> MACAAARSPAEQDRFICIYPAYLNNKKTIAEGRRIPISKAVENPTATEIQDVCSAVGLNVFLEKNKMYSREWNRDVQYRGRVRVQLKQEDGSLCLVQFPSRKSVMLYAAEMIPKLKTRTQKTGGGDQSLQQGEGSKKGKGKKKK;> MASADSRRLGDGDGAGGAFQPYLDSLRQELQQRDPTVLSVVVALLAVLLTLVFWKLVRSRRSSQRAVLLLGLCDSGKTLLFVRLLTGHYRDTQTSITDSSATYRVNNNRGNSLTLIDLPGHESLRLQFLERFKTSARAVVFVVDSAAFQREVKDVAEFLYQVLIDSMSLKNTPSFLIACNKQDIAMAKSAKLIQQQLEKELNTLRVTRSAAPSTLDSSSTAPAQLGKKGKEFEFSQLPLKVEFLECSAKGGRGDPGSADIQDLEKWLAKIA;> MVLADLGRKITSALRSLSNATIINEEVLNAMLKEVCTALLEADVNIKLVKQLRENVKSAIDLEEMASGLNKRKMIQHAVFKELVKLVDPGVKAWTPTKGKQNVIMFVGLQGSGKTTTCSKLAYYYQRKGWKTCLICADTFRAGAFDQLKQNATKARIPFYGSYTEMDPVIIASEGVEKFKNENFEIIIVDTSGRHKQEDSLFEEMLQVANAIQPDNIVYVMDASIGQACEAQAKAFKDKVDVASVIVTKLDGHAKGGGALSAVAATKSPIIFIGTGEHIDDFEPFKTQPFISKLLGMGDIEGLIDKVNELKLDDNEALIEKLKHGQFTLRDMYEQFQNIMKMGPFSQILGMIPGFGTDFMSKGNEQESMARLKKLMTIMDSMNDQELDSTDGAKVFSKQPGRIQRVARGSGVSTRDVQELLTQYTKFAQMVKKMGGIKGLFKGGDMSKNVSQSQMAKLNQQMAKMMDPRVLHHMGGMAGLQSMMRQFQQGAAGNMKGMMGFNNM;> MLDFFTIFSKGGLVLWCFQGVSDSCTGPVNALIRSVLLQERGGNNSFTHEALTLKYKLDNQFELVFVVGFQKILTLTYVDKLIDDVHRLFRDKYRTEIQQQSALSLLNGTFDFQNDFLRLLREAEESSKIRAPTTMKKFEDSEKAKKPVRSMIETRGEKPKEKAKNSKKKGAKKEGSDGPLATSKAVPAEKSGLPVGPENGVELSKEELIRRKREEFIQKHGRGLEKSSKSKSEAPKEKGKKAPRVWELGGCANKEVLDYSTPTTNGAPEAALSEDINLIRGTGPGGQLQDLDCSSSDDEGAAQNSTKPSSTKGTLGGMFGMLKGLVGSKSLSREDMESVLDKMRDHLIAKNVAADIAVQLCESVANKLEGKVMGTFSTVTSTVKQALQESLVQILQPQRRVDMLRDIMDAQRRQRPYVVTFCGVNGVGKSTNLAKISFWLLENGFSVLIAACDTFRAGAVEQLRTHTRRLSALHPPEKHGGRTMVQLFEKGYGKDAAGIAMEAIAFARNQGFDVVLVDTAGRMQDNAPLMTALAKLITVNTPDLVLFVGEALVGNEAVDQLVKFNRALADHSMAQTPRLIDGIVLTKFDTIDDKVGAAISMTYITSKPIVFVGTGQTYCDLRSLNAKAVVAALMKA;> MASGGSGGVSVPALWSEVNRYGQNGDFTRALKTVNKILQINKDDVTALHCKVVCLIQNGSFKEALNVINTHTKVLANNSLSFEKAYCEYRLNRIENALKTIESANQQTDKLKELYGQVLYRLERYDECLAVYRDLVRNSQDDYDEERKTNLSAVVAAQSNWEKVVPENLGLQEGTHELCYNAACALIGQGQLSQAMKILQKAEDLCRRSLSEDSDGTEEDPQAELAIIHGQMAYILQLQGRTEEALQLYNQIIKLKPTDVGLLAVIANNIITINKDQNVFDSKKKVKLTNAEGVEFKLSKKQLQAIEFNKALLAMYTNQAEQCRKISASLQSQSPEHLLPVLIQAAQLCREKQHTKAIELLQEFSDQHPENAAEIKLTMAQLKISQGNISKACLILRSIEELK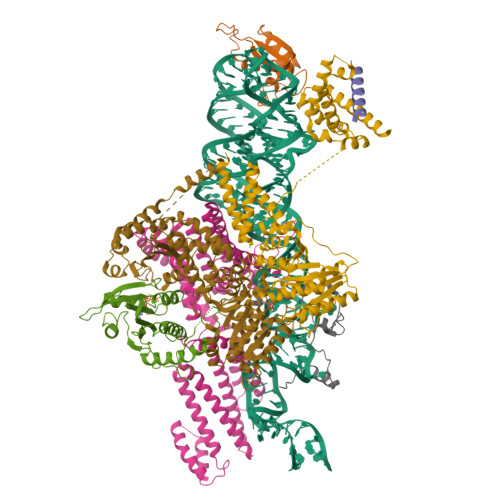HKPGMVSALVTMYSHEEDIDSAIEVFTQAIQWYQNHQPKSSAHLSLIREAANFKLKYGRKKEAISDLEQLWKQNPKDIHTLAQLISAYSLVDPEKAKALSKHLPSSDSMSLKVDVEALENSPGATYIRKKGGKVAGDSQPKEQGQGDLKKKKKKKKGKLPKNYDPKVTPDPERWLPMRERSYYRGRKKGKKKDQIGKGTQGATAGASSELDASKTVSSPPTSPRPGSAATASASTSNIIPPRHQKPAGAPATKKKQQQKKKKGGKGGW> PIEESLAAVIPISHLGEVGKWANNVLNCTEYSEKKIAERLYVFITFLTDMGVLEKINNLYKPANLKFQKALGLHDKQLTEETVSLTLNEYVLPTVSKYSDKIKSPESLYLLSSLRLLLNSLNALKLINEKSTHGKIDELTYIELSAAAFNGRHLKNIPRIPIFCILYNILTVMSENLKTESLFCGSNQYQYYWDLLVIVIAALETAVTKDEARLRVYKELIDSWIASVKSKSDIEITPFLNINLEFTDVLQLSRGHSITLLWDIFRKNYPTTSNSWLAFEKLINLSEKFDKVRLLQFSESYNSIKDLMDVFRLLNDDVLNNKLSEFNLLLSKLEDGINELELISNKFLNKRKHYFADEFDNLIRYTFSVDTAELIKELAPASSLATQKLTKLITNKYNYPPIFDVLWTEKNAKLTSFTSTIFSSQFLEDVVRKSNNLKSFSGNQIKQSISDAELLLSSTIKCSPNLLKSQMEYYKNMLLSWLRKVIDIHVGGDCLKLTLKELCSLIEEKTASETRVTFAEYIFPALDLAESSKSLEELGEAWITFGTGLLLLFVPDSPYDPAIHDYVLYDLFLKTKTFSQNLMKSWRNVRKVISGDEEIFTEKLINTISDDDAPQSPRVYRTGMSIDSLFDEWMAFLSSTMSSRQIKELVSSYKCNSDQSDRRLEMLQQNSAHFLNRLESGYSKFADLNDILAGYIYSINFGFDLLKLQKSKDRASFQISPLWSMDPINISCAENVLSAYHELSRFFKKGDMEDTSIEKVLMYFLTLFKFHKRDTNLLEIFEAALYTLYSRWSVRRFRQEQEENEKSNMFKFNDNSDDYEADFRKLFPDYEDTALVTNEKDISSPENLDDIYFKLADTYISVFDKDHDANFSSELKSGAIITTILSEDLKNTRIEELKSGSLSAVINTLDAETQSFKNTEVFGNIDFYHDFSIPEFQKAGDIIETVLKSVLKLLKQWPEHATLKELYRVSQEFLNYPIKTPLARQLQKIEQIYTYLAEWEKYASSEVSLNNTVKLITDLIVSWRKLELRTWKGLFNSEDAKTRKSIGKWWFYLYESIVISNFVSEKKETAPNATLLVSSLNLFFSKSTLGEFNARLDLVKAFYKHIQLIGLRSSKIAGLLHNTIKFYYQFKPLIDERITNGKKSLEKEIDDIILLASWKDVNVDALKQSSRKSHNNLYKIVRKYRDLLNGDAKTIIEAGLLYXXXXXXXXXXXXXXXXXXXXXXXXXXXXXXXRNIDTVASNMDSYLEKISSQEFPNFADLASDFYAEAERLRKETPNVYTKENKKRLAYLKTQKSKLLGDALKELRRIGLKVNFREDIQKVQSSTTTILANIAPFNNEYLNSSDAFFFKILDLLPKLRSAASNPSDDIPVAAIERGMALAQSLMFSLITVRHPLSEFTNDYCKINGMMLDLEHFTCLKGDIVHSSLKANVDNVRLFEKWLPSLLDYAAQTLSVISKYSATSEQQKILLDAKSTLSSFFVHFNSSRIFDSSFIESYSRFELFINELLKKLENAKETGNAFVFDIIIEWIKANKGGPIKKEQKRGPSVEDVEQAFRRTFTSIILSFQKVIGDGIESISETDDNWLSASFKKVMVNVKLLRSSVVSKNIETALSLLKDFDFTTTESIYVKSVISFTLPVITRYYNAMTVVLERSRIYYTNTSRGMYILSTILHSLAKN

The AAA+ (ATPases Associated with various cellular Activities) family member Rea1 (or Midasin) consists of nearly 5000 amino acids and generates force to mechanically remove assembly factors. Rea1 consists of an N-terminal α-helical domain (NTD), a ring of six AAA+ domains, and the C-terminal tail. The Rea1 tail is subdivided into an α-helical linker region, a D/E-rich region, and a MIDAS (Metal-Ion-Dependent Adhesion Site) domain which is responsible for the interaction with the Ytm1 and Rsa4 substrates. Rea1 pulls out the Ytm1 complex to promote the transfer of pre-60S particles from the nucleolus to the nucleoplasm.

The Rea1 linker map revealed side-chains throughout. In addition to the stem and middle domain, the Rea1 linker also comprises three α-helical bundles at its top (top1-top3). The linker emerges at an angle of roughly 120° from the AAA+ ring. The 210 Å length of the complete linker fits well with the ~200 Å AAA+ ring extension that bends towards the pre-60S particle when Rea1 is bound to it, suggesting that the linker is a key element for Rea1 tail remodelling. Comparing 2D projections of our Rea1 structure to this data suggests the pivot point area is located in the region between middle and stem domains of the linker. The horseshoe-like arrangement of the three linker top domains is stabilised by the middle domain. The various interactions of top1 hold this domain in a strained conformation as indicated by a long, bent α-helix. The connection between the top1 and the top2 domains is established via an extended ~40 aa peptide region between them, which could provide flexibility during linker remodelling. The top3 domain is a four α-helix bundle insertion into the linker top2 domain, and it connects this domain back to the globular extension of the linker middle domain. The D/E-rich region and the MIDAS domain that follows are not resolved.> NKKTAQLLHADTPRLVTWDAGLCTSFKIVPIVPAQVPQDVLAYTFFTSSYAIQSPFPEAAVSRIVVHTRWASNVDFDRDSSVIMAPPTENNIHLFKQLLNTETLSVRGANPLMFRANVLHMLLEFVLDNLYLNRHTGFSQDHTPFTEGANLRSLPGPDAEKWYSIMYPTRMGTPNVSKICNFVASCVRNRVGRFDRAQMMNGAMSEWVDVFETSDALTVSIRGRWMARLARMNINPTEIEWALTECAQGYVTVTSPYAPSVNRLMPYRISNAERQISQIIRIMNIGNNATVIQPVLQDISVLLQRISPLQIDPTIISNTMSTVSESTTQTLSPASSILGKLRPSNSDFSSFRVALAGWLYNGVVTTVIDDSSYPKDGGSVTSLENLWDFFILALALPLTTDPCAPVKAFMTLANMMVGFETIPMDNQIYTQSRRASAFSTPHTWPRCFMNIQLISPIDAPILRQWAEIIHRYWPNPSQIRYGAPNVFGSANLFTPPEVLLLPIDHQPANVTTPTLDFTNELTNWRARVCELMKNLVDNQRYQPGWTQSLVSSMRGTLDKLKLIKSMTPMYLQQLAPVELAVIAPMLPFPPFQVPYVRLDRDRVPTMVGVTRQSRDTITQPALSLSTTNTTVGVPLALDARAITVALLSGKYPPDLVTNVWYADAIYPMYADTEVFSNLQRDMITCEAVQTLVTLVAQISETQYPVDRYLDWIPSLRASAATAATFAEWVNTSMKTAFDLSDMLLEPLLSGDPRMTQLAIQYQQYNGRTFNVIPEMPGSVIADCVQLTAEVFNHEYNLFGIARGDIIIGRVQSTHLWSPLAPPPDLVFDRDTPGVHIFGRDCRISFGMNGAAPMIRDETGMMVPFEGNWIFPLALWQMNTRYFNQQFDAWIKTGELRIRIEMGAYPYMLHYYDPRQYA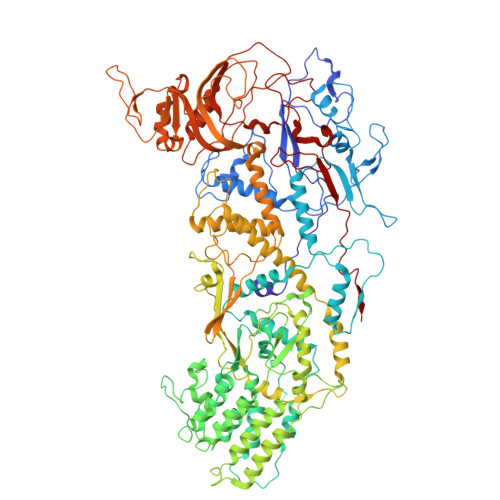NAWNLTSAWLEEITPTSIPSVPFMVPISSDHDISSAPAVQYIISTEYNDRSLFCTNSSSPQTIAGPDKHIPVERYNILTNPDAPPTQIQLPEVVDLYNVVTRYAYETPPITAVVMGVP>DPFTMLQIEFITDLGARVTVNVEHESRLLDVQRHYGRLGWTSGEIPSGGYQFPIENEADFDWSLIGARKWKSPEGEELVIHRG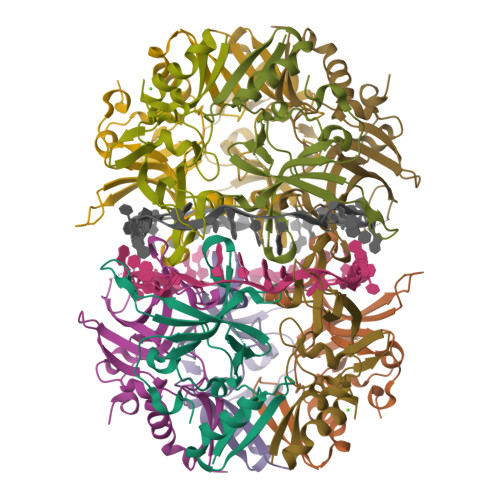HAYRRRELEAVDSRKLKLPAAIKYSRGAKVSDPQHVREKADGDIEYVSLAIFRGGKRQERYAVPG[5x]> MAGGLSQLVAYGAQDVYLTGNPQITFFKTVYRRYTNFAIESIQQTINGSVGFGNKVSTQISRNGDLITDIVVEFVLTKGGNGGTTYYPAEELLQDVELEIGGQRIDKHYNDWFRTYDALFRMNDDRYNYRRMTDWVNNELVGAQKRFYVPLIFFFNQTPGLALPLIALQYHEVKLYFTLASQVQGVNYNGSSAIAGAAQPTMSVWVDYIFLDTQERTRFAQLPHEYLIEQLQFTGSETATPSATTQASQNIRLNFNHPTKYLAWNFNNPTNYGQYTALANIPGACSGAGTAAATVTTPDYGNTGTYNEQLAVLDSAKIQLNGQDRFATRKGSYFNKVQPYQSIGGVTPAGVYLYSFALKPAGRQPSGTCNFSRIDNATLSLTYKTCSIDATSPAAVLGNTETVTANTA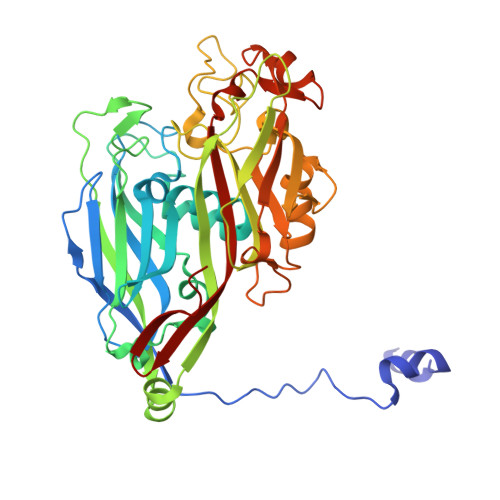TLLTALNIYAKNYNVLRIMSGMGGLAYAN>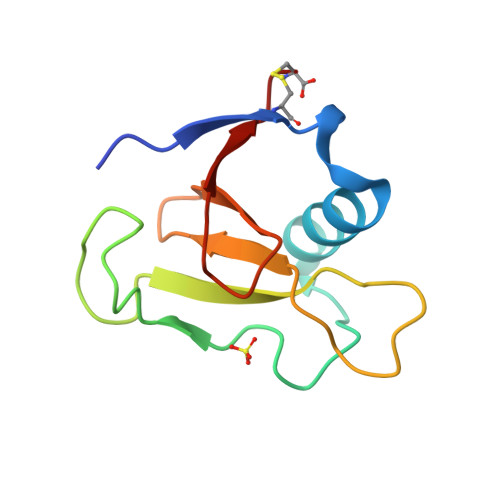[3x]ADPALADVCRTKLPSQAQDTLALIAKNGPYPYNRDGVVFENRESRLPKKGNGYYHEFTVVTPGSNDRGTRRVVTGGYGEQYWSPDHYATFQEIDPRC> GSAKDPLNFIKTISPIQKINFNGFEFYIKRDDLLGEINGNKARKLAF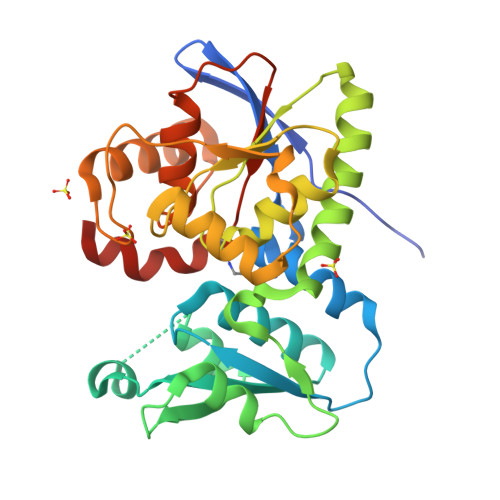YIHQRYPKNQSFVSYGGSQSNALAALSIFAKQRSYKLVFACEKISTFLKNNPCGNYALALENGVDFVENIHSLSLKQFALSLCKKDDVFIEQGIANLEAQYGYMELAQEIQMQSQSLKLDFDIFLPSGTGTSAAFLAKYSKFKVFTCACVGDIKYLKKQILTLDPSYDFSNLEFLTSDKKYHFAKPYKEFYELYMDLKLKCNIEFDLLYDILGLSIALKQEWKKPLLYIHQGGILGNSTMLERYKFKKSV>[4x]MGSSHHHHHHSSENLYFQGHMWNSRKVGVLGGGQLGRMLVESANRLNIQVNVLDADNSPAKQISAHDG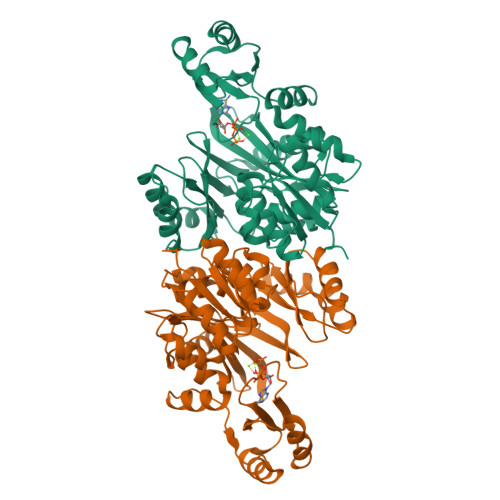HVTGSFKEREAVRQLAKTCDVVTAEIEHVDTYALEEVASEVKIEPSWQAIRTIQNKFNQKEHLRKYGIPMAEHRELVENTPAELAKVGEQLGYPLMLKSKTMAYDGRGNFRVNSQDDIPEALEALKDRPLYAEKWAYFKMELAVIVVKTKDEVLSYPTVETVQEDSICKLVYAPARNVSDAINQKAQELARKAVAAFDGKGVFGVEMFLLEDDSIMLCEIASRIHNSGHYTIEGCALSQFDAHLRAILDLPIPAQSLEIRQPSIMLNIIGGAAPDTHLQAAECALSIPNASIHLYSKGAAKPGRKMGHITVTAPTMHEAETHIQPLIDVVDRIRA>GFLSGKRILVTGVASKLSIAYGIAQAMHREGAELAFTYQNDKLKGRVEEFAAQLGSDIVLQCDVAEDASIDTMFAELGKVWPKF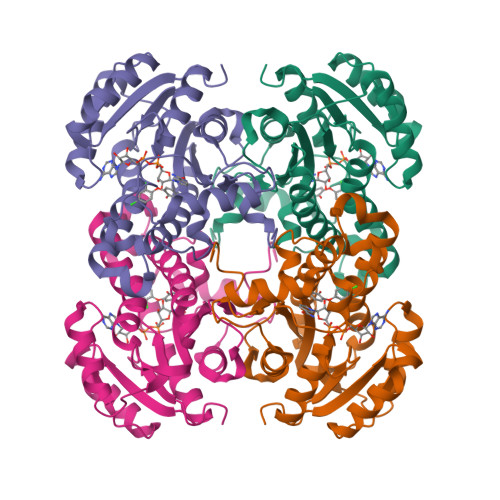DGFVHSIGFAPGDQLDGDYVNAVTREGFKIAHDISSYSFVAMAKACRSMLNPGSALLTLSYLGAERAIPNYNVMGLAKASLEANVRYMANAMGPEGVRVNAISAGPIRTLAASGIKDFRKMLAHCEAVTPIRRTVTIEDVGNSAAFLCSDLSAGISGEVVHVDGGFSIAAMNELELK[2x]>[2x]GPLGSPEFETAGTVDLDAPVQKDTAMSLVSSFENSSTDWQ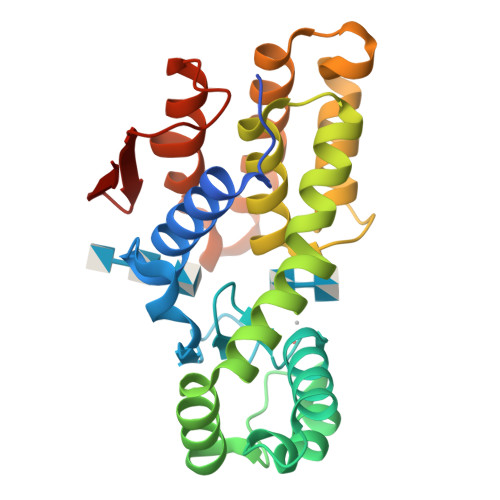AQYGYLEDIAAGRGYTGGLIGFTSGTGDMLELVRAYSASSPGNPLEQYIPALEAVNGTDSHAGLGQGFEQAWADAAETSEFRAAQDAERDRVYFDPAVAQGKADGLSALGQFAYYDTLVVHGPGSQRDAFGGIRAEALSAALPPSQGGDETEYLEAFFDARNVIMREEPAHADTSRIDTAQRVFLQNGNFDLERPLTWSVYGDQYSLN5'-O-[(R)-(3-aminopropoxy)(L-alpha-aspartylamino)phosphoryl]adenosine | C17 H27 N8 O9 P | 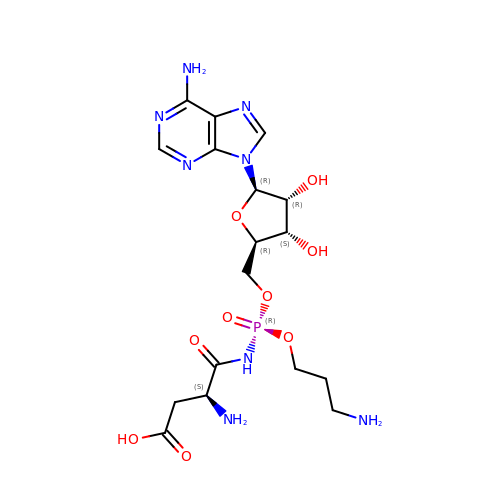CBRVFFLBHDTTIM-FGNORGMNSA-N> GPVCAEASDVYSPCMIASTPPAPFSDVTAVTFDLINGKITPVGDDNWNTHIYNPPIMNVLRTAAWKSGTIHVQLNVRGAGVKRADWDGQVFVYLRQSMNPESYDAR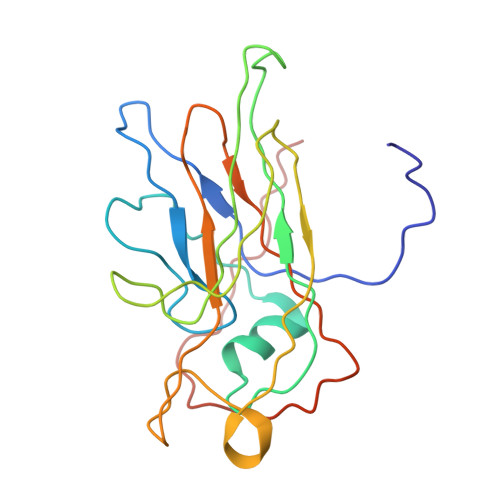TFVISQPGSAMLNFSFDIIGPNSGFEFAESPWANQTTWYLECVATNPRQIQQFEVNMRFDPNFRVAGNILMPPFPLSTETPPL(5R)-3,5-bis(4-chlorobenzyl)-4-(6-chloro-1H-indol-3-yl)-5-hydroxyfuran-2(5H)-one 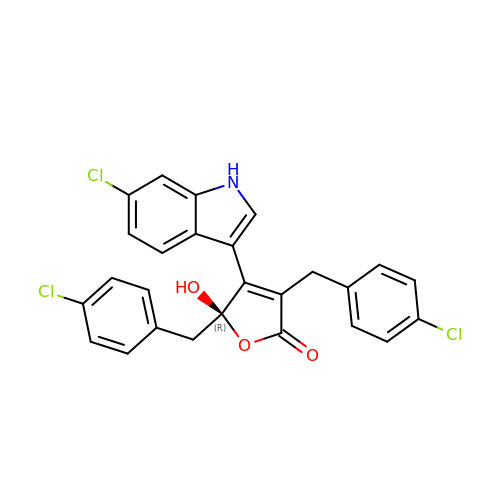| C26 H18 Cl3 N O3 | MLBSWDQJORDIOB-AREMUKBSSA-N> MGAEEESTAILYPFTISGNDRNGNFTINFKGTPNSTNNGCIGYSYNGDWEKIEWEGSCDGN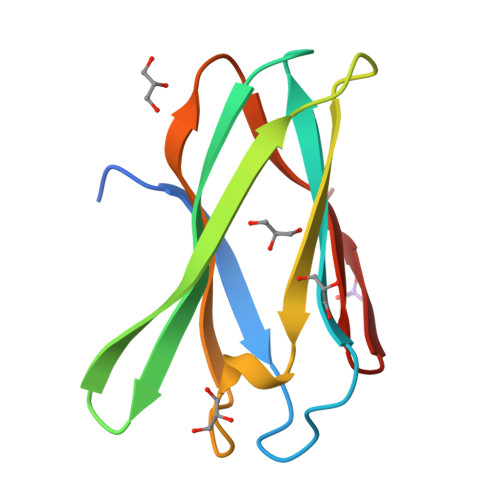GNLVVEVPMSKIPAGVTSGEIQIWWHSGDLKMTDYKALEHHHHHH> SPIFQGGSYQLNNKSIDISSLLLDKLSGESQTVVMKFKADKPNSLQALFGLSNSKAGFKNNYFSIFMRDSGEIGVEIRDAQKGINYLFSRPASLWGKHKGQAVEN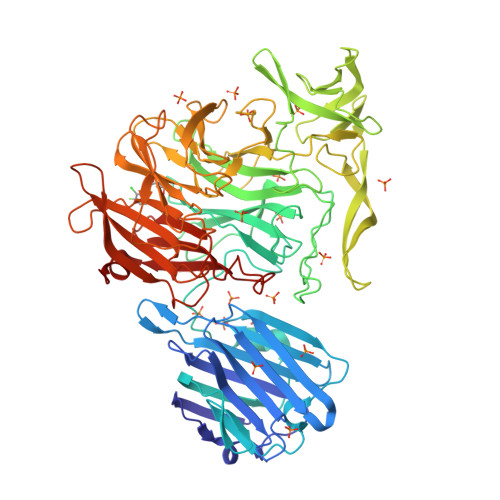TLVFVSDSKDKTYTMYVNGIEVFSETVDTFLPISNINGIDKATLGAVNREGKEHYLAKGSIDEISLFNKAISDQEVSTIPLSNPFQLIFQSGDSTQANYFRIPTLYTLSSGRVLSSIDARYGGTHDSKSKINIATSYSDDNGKTWSEPIFAMKFNDYEEQLVYWPRDNKLKNSQISGSASFIDSSIVEDKKSGKTILLADVMPAGIGNNNANKADSGFKEINGHYYLKLKKNGDNDFRYTVRENGVVYNETTNKPTNYTINDKYEVLEGGKSLTVEQYSVDFDSGSLRERHNGKQVPMNVFYKDSLFKVTPTNYIAMTTSQNRGESWEQFKLLPPFLGEKHNGTYLCPGQGLALKSSNRLIFATYTSGELTYLISDDSGQTWKKSSASIPFKNATAEAQMVELRDGVIRTFFRTTTGKIAYMTSRDSGETWSKVSYIDGIQQTSYGTQVSAIKYSQLIDGKEAVILSTPNSRSGRKGGQLVVGLVNKEDDSIDWKYHYGIDLPSYGYAYSAITELPNHHIGVLFEKYDSWSRNELHLSNVVQYIDLEINDLTKLE4-(1,4'-bipiperidin-1'-yl)-7-({5-chloro-2-[(2-methoxyphenyl)amino]pyrimidin-4-yl}amino)-2-methyl-2,3-dihydro-1H-isoindol-1-one 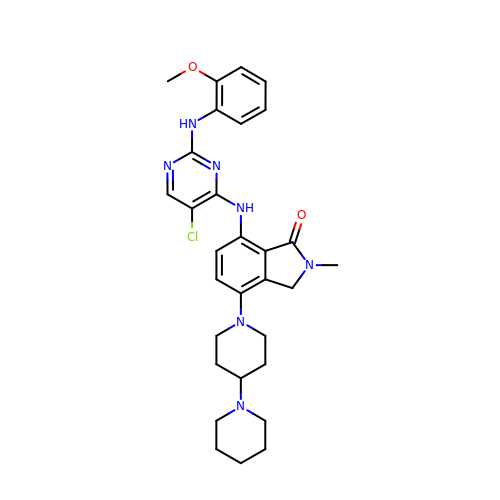| C30 H36 Cl N7 O2 | CXZCUCWQLXRDJA-UHFFFAOYSA-N1-CYCLOHEXYL-N-{[1-(4-METHYLPHENYL)-1H-INDOL-3-YL]METHYL}METHANAMINE | C23 H28 N2 | 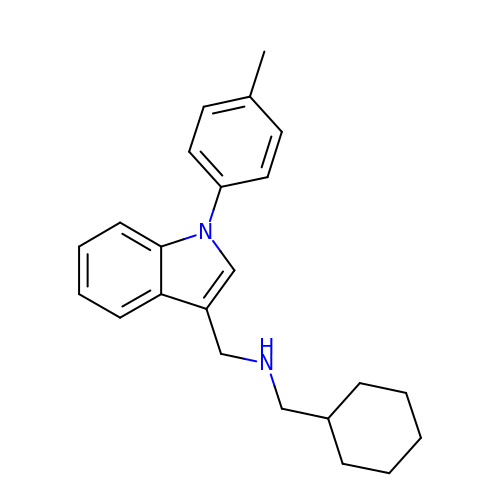MMIJMYOYKAKQPN-UHFFFAOYSA-N> MALTTTGTEQHDLFSGTFWQNPHPAYAALRAEDPVR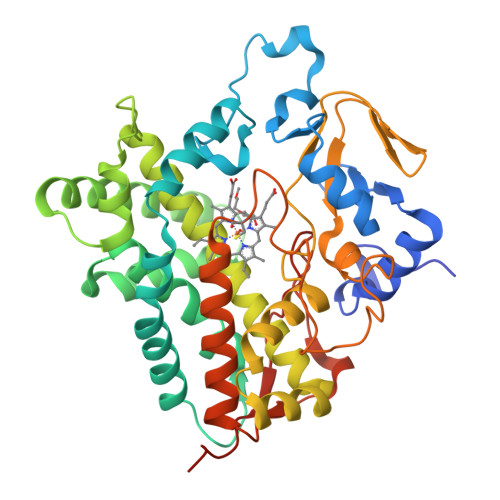KLALPDGPVWLLTRYADVREAFVDPRLSKDWRHTLPEDQRADMPATPTPMMILMDPPDHTRLRKLVGRSVTVRRMNELEPRITEIADGLLAGLPTDGPVDLMREYAFQIPVQVICELLGVPAEDRDDFSAWSSVLVDDSPADDKNAAMGKLHGYLSDLLERKRTEPDDALLSSLLAVSDEDGDRLSQEELVAMAMLLLIAGHETTVNLIGNGVLALLTHPDQRKLLAEDPSLISSAVEEFLRFDSPVSQAPIRFTAEDVTYSGVTIPAGEMVMLGLAAANRDADWMPEPDRLDITRDASGGVFFGHGIHFCLGAQLARLEGRVAIGRLFADRPELALAVGLDELVYRESTLVRGLSRMPVTMGPRSALEHHHHHH> SSQIRQNYSTEVEAAVNRLVNLYLRASYTYLSLGFYFDRDDVALEGVCHFFRELAEEKREGAERLLKMQNQRGGRALFQDLQ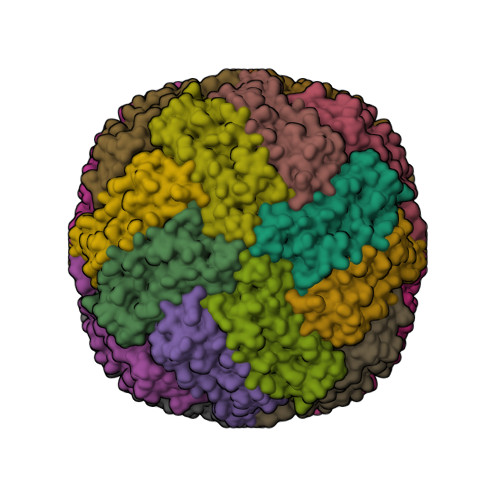KPSQDEWGTTLDAMKAAIVLEKSLNQALLDLHALGSAQADPHLCDFLESHFLDEEVKLIKKMGDHLTNIQRLVGSQAGLGEYLFERLTLK> MQKDLKMPSTANAKLNEQGEISADIGGIAVSVHAQSCTEDSPGIMLCNRSPVVEVTFPGAKPIALEPEALYVDSNSTFYHGPLDDTYKKNRHSIILTDINGDGHEDVVVWSGKEGNYGGPSYSVYLFDA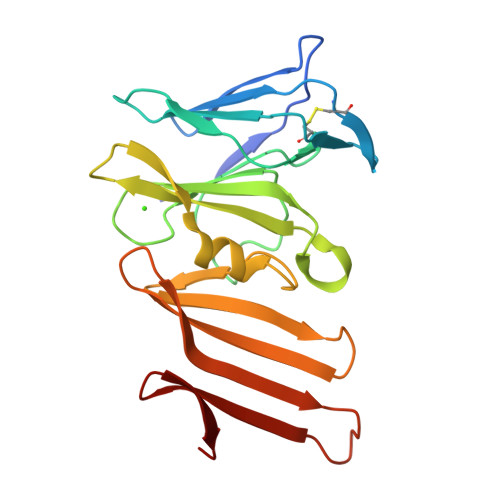AQKTLVFNQSLSDITVMANGLFSVKGNMLTSTSGDGCCIHVFDTYELKNNEAVLIERLTEDTNDPANPKKKIERLQDGEMKEVSN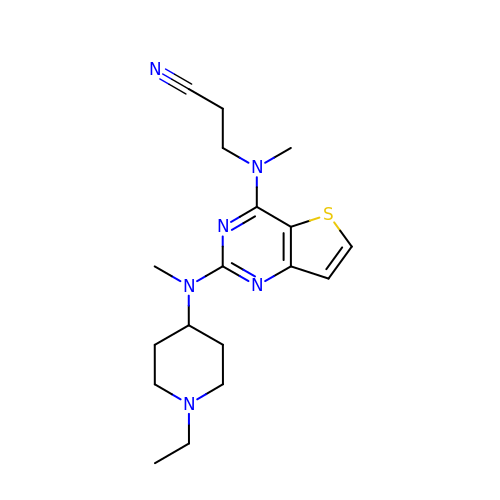3-[[2-[(1-ethylpiperidin-4-yl)-methyl-amino]thieno[3,2-d]pyrimidin-4-yl]-methyl-amino]propanenitrile | C18 H26 N6 S | MLPWBUBDJOKZOR-UHFFFAOYSA-N> GSHMLSYRHSFHAGNHADVLKHTVQSLIIESLKEKDKPFLYLDTHAGAGRYQLGSEHAERTGKYLEGIARIWQQDDLPAELEAYINVVKHFNRSGQLRYYPGSPLIARQLLREQDSLQLTELHPSDYPLLRSEFQKDSRARVEKADGFQQLKAKLPPVSRRGLILIDPPYEMKTDYQAVVSGIAEGYKRFATGTYALWYPVVLRQQIKRMIHDLEATGIRKILQIELAVLPDSDRRGMTASGMIVINPPWKLEQQMNNVLPWLHSKLVP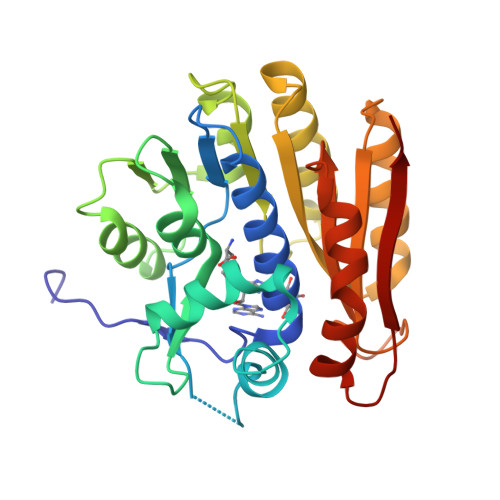AGTGHATVSWIVPE>[6x]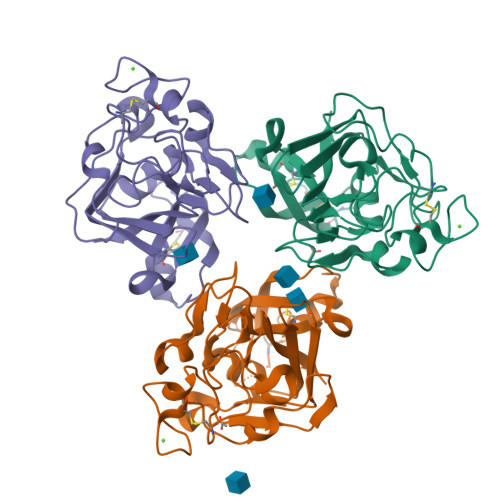PQPCLTGPRTCKDLLDRGHFLSGWHTIYLPDCRPLTVLCDMDTDGGGWTVFQRRVDGSVDFYRDWATYKQGFGSRLGEFWLGNDNIHALTAQGTSELRTDLVDFEDNYQFAKYRSFKVADEAEKYNLVLGAFVEGSAGDSLTFHNNQSFSTKDQDNDLNTGNCAVMFQGAWWYKNCHTSNLNGRYLRGTHGSFANGINWKSGKGYNYSYKVSEMKVRPA6-({[(1R,3S)-3-(aminomethyl)cyclohexyl]methyl}amino)pyridine-3-carboxamide | C14 H22 N4 O | 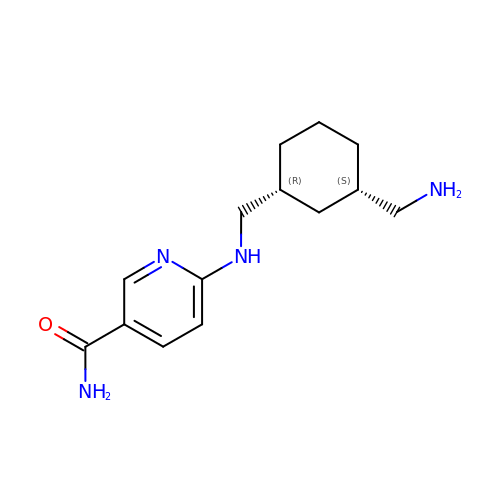UUTSJGSKPMLQOF-WDEREUQCSA-N> MAVDSSNSATGPMRVFAIGNPILDLVAEVPSSFLDEFFLKRGDATLATPEQMRIYSTLDQFNPTSLPGGSALNSVRVVQKLLRKPGSAGYMGAIGDDPRGQVLKELCDKEGLATRFMVAPGQSTGVCAVLINEKERTLCTHLGACGSFRLPEDWTTFASGALIFYATAYTLTATPKNAFEVAGYAHGIPNAIFTLNLSAPFCVELYKDAMQSLLLHTNILFGNEEEFAHLAKVHNLVAAEKTALSTANKEHAVEVCTGALRLLTAGQNTGATKLVVMTRGHNPVIAAEQTADGTVVVHEVGVPVVAAEKIVDTNGAGDAFVGGFLYALSQGKTVKQCIMCGNACAQDVIQHVG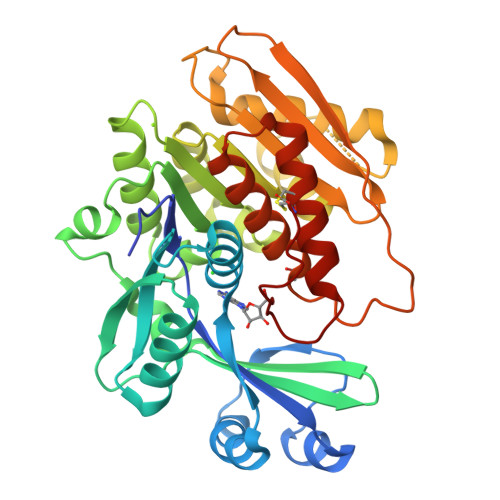FSLSFTSLPC> MLSPEALTTAVDAAQQAIALADTLDVLARVKTEHLGDRSPLALARQALAVLPKEQRAEAGKRVNAARNAAQRSYDERLATLRAERDAAVLVAEGIDVTLPSTRVPAGARHPIIMLAEHVADTFIAMGWELAEGPEVETEQFNFDALNFPADHPARGEQDTFYIAPEDSRQLLRTHTSPVQIRTLLARELPVYIISIGRTFRTDELDATHTPIFHQVEGLAVDRGLSMAHLRGTLDAFARAEFGPSARTRIRPHFFPFTEPSAEVDVWFANKIGGAAWVEWGGCGMVHPNVLRATGIDPDLYSGFAFGMGLERTLQFRNGIPDMRDMVEGDVRFSLPFGVGA;> QSNAMRLPYSWLREVVAVGASGWDVTPGELEQTLLRIGHEVEEVIPLGPVDGPVTVGRVADIEELTGYKKPIRACAVDIGDRQYREIICGATNFAVGDLVVVALPGATLPGGFTISARKAYGRNSDGMICSAAELNLGADHSGILVLPPGAAEPGADGAGVLGLDDVVFHLAITPDRGYCMSVRGLARELACAYDLDFVDPASNSRVPPLPIEGPAWPLTVQPETGVRRFALRPVIGIDPAAVSPWWLQRRLLLCGIRATCPAVDVTNYVMLELGHPMHAHDRNRISGTLGVRFARSGETAVTLDGIERKLDTADVLIVDDAATAAIGGVMGAASTEVRADSTDVLLEAAIWDPAAVSRTQRRLHLPSEAARRYERTVDPAISVAALDRCARLLADIAGGEVSPTLTDWRGDPPCDDWSPPPIRMGVDVPDRIAGVAYPQGTTARRLAQIGAVVTHDGDTLTVTPPSWRPDLRQPADLVEEVLRLEGLEVIPSVLPPAPAGRGLTAGQQRRRTIGRSLALSGYVEILPTPFLPAGVFDLWGLEADDSRRMTTRVLNPLEADRPQLATTLLPALLEALVRNVSRGLVDVALFAIAQVVQPTEQTRGVGLIPVDRRPTDDEIAMLDASLPRQPQHVAAVLAGLREPRGPWGPGRPVEAADAFEAVRIIARASRVDVTLRPAQYLPWHPGRCAQVFVGESSVGHAGQLHPAVIERSGLPKGTCAVE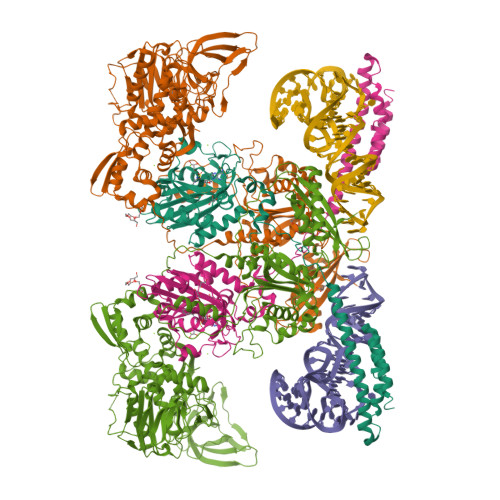LNLDAIPCSAPLPAPRVSPYPAVFQDVSLVVAADIPAQAVADAVRAGAGDLLEDIALFDVFTGPQIGEHRKSLTFALRFRAPDRTLTEDDASAARDAAVQSAAERVGAVLRG> MEGERKNNNKRWYFTREQLENSPSRAFGVDPDKELSYRQQAANLLQDMGQRLNVSQLTINTAIVYMHRFYMIQSFTRFPGNSVAPAALFLAAKVEGQPKKLEHVIRVAHTCLHPQESLPDTRSEAYLQQVQDLVILESIILQTLGFELTIDHPHTHVVKCTQLVRASKDLAQT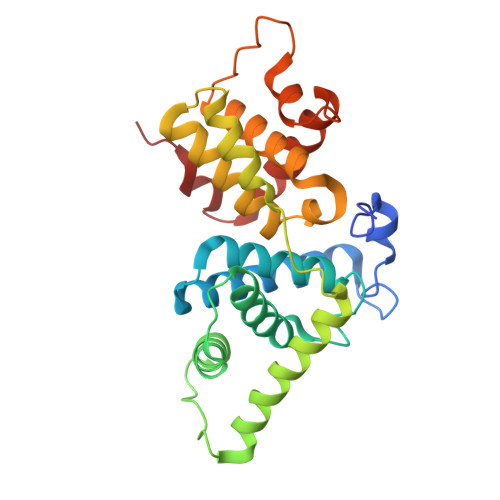SYFMATNSLHLTTFSLQYTPPVVACVCIHLACKWSNWEIPVSTDGKHWWEYVDATVTLELLDELTHELLQILEKTPNRLKRIWNWR> MSTAITRQIVLDTETTGMNQIGAHYEGHKIIEIGAVEVVNRRLTGNNFHVYLKPDRLVDPEAFGVHGIADEFLLDKPTFAEVADEFMDYIRGAELVIHNAAFDIGFMDYEFSLLKRDIPKTNTFCKVTDSLA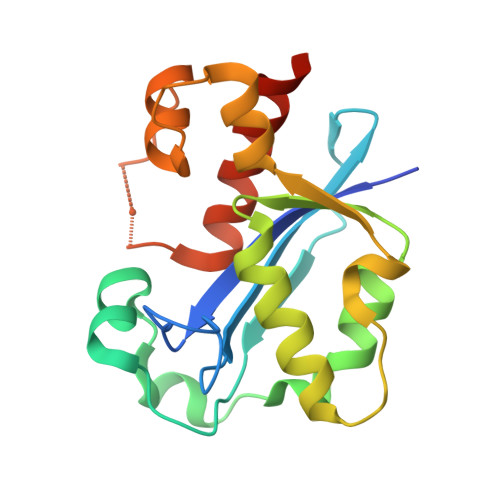VARKMFPGKRNSLDALCARYEIDNSKRTLHGALLDAQILAEVYLAMTGGQTSMA> ADPSERCDDWGLDTMRQIQVFEDEPARIKCPLFEHFLKFNYSTAHSAGLTLIWYWTRQDRDLEEPINFRLPENRISKEKDVLWFRPTLLNDTGNYTCMLRNTTYCSKVAFPLEVVQKDSCFNSPMKLPVHKLYIEYGIQRITCPNVDGYFPSSVKPTITWYMGCYKIQNFNNVIPEGMNLSFLIALISNNGNYTCVVTYPENGRTFHLTRTLTVKVVGSPKNAVPPVIHSPNDHVVYEKEPGEELLIPCTVYFSFLMDSRNEVWWTIDGKKPDDI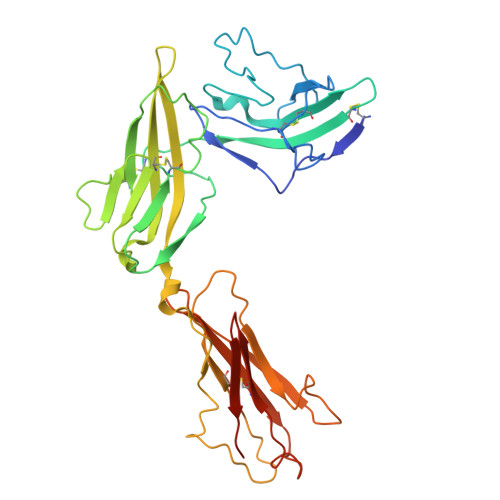TIDVTINESISHSRTEDETRTQILSIKKVTSEDLKRSYVCHARSAKGEVAKAAKVKQKHHHHHH> MGQYKKLWYLLFAVLAVCFTILGYMGSEVYKKAPPYPEQVVSASGKVLMAKDDILAGQSAWQTTGGMEVGSVLGHGAYQAPDWTADWLHRELSAWLDLTAQQTYGKKFDEVSPEEQAVLKTRLADEYRNQSRIKEDGSVVISDTRVKAIESILPYYHGVYGDDPALQTTREHFAMKNNTLPSQEAREKLFDFFFWTSWSASTNRPDETFTYTNNWPHEPLINNVPTTENYMWSFTSVVLLLMGIGLLMWGYSFLTKHEEVEVPTEDPISKVQLTPSQKALGKYVFLTVALFVVQVLLGGLTAHYTVEGQGFYGIDEALGFEMSDWFPYALTRTWHIQSAIFWIATGFLTAGLFLAPIVNGGKDPKFQRAGVNFLYIALFIVVGGSYAGNFFALTHILPPEFNFWFGHQGYEYLDLGRFWQLLLMVGLLLWLFLMLRCTVSAFKEKGVDKNLLAIFVASMVGVGVFYAPGLFYGEKSPIAVMEYWRWWVVHLWVEGFFEVFATAAFAFVFYNMGFVRRSTATASTLAAAAIFMLGGVPGTLHHLYFSGSTSASMAIGACFSALEVVPLVLLGREA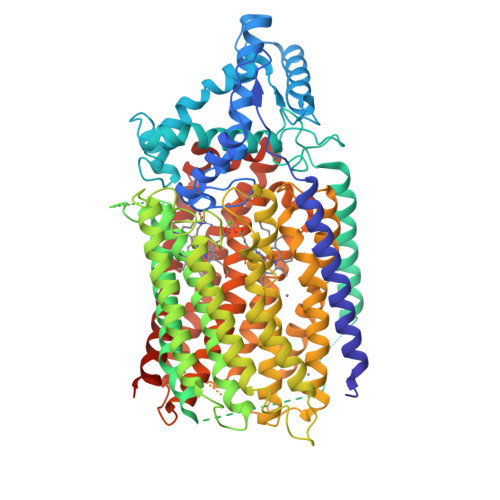YEHWSYQHLSEWAKRLRWPLMCFVAVAFWNMIGAGVFGFLINPPISLFYIQGLNTSAVHAHAALFGVYGFLALGFVLLVARYLKPNVQFDDKLMTWGFWLLNGGLVGMIAISLLPVGVIQAYASITHGLWYARSEEFLQMEILDTLRWVRTAADLIFIGGAICVAIQATKIVFGRDK>[2x]SEKYDGEWNEGRMQGWGKYFYADGGVYEGEWVDGRMHGRGTYVFPNGNKYEGEWVEDRKDGY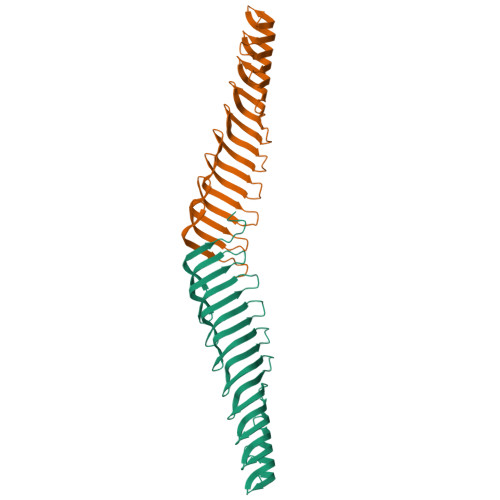GILLYTNGERYEGYWHLDKAHGKGTLTFLQGDRYVGEWHYGKKHGHGVLSYSNGDTYDGEWRDDDAWGYGVLQYANGCRYEGEWAEDRRHGKGLLVLPDGSSYEGSFAHGKKDGPGKIILKDGSMYIGTWKDGVIVGQGEFRLSENCDLSNPDY> IDHKSKYLREAALEANLSHPETTPTMLTCPIDSGFLKDPVITPEGFVYNKSSILKWLETKKEDPQSRKPLTAKDLQPFPELLIIVNRFVETQTNYEKLKNRLVQNAR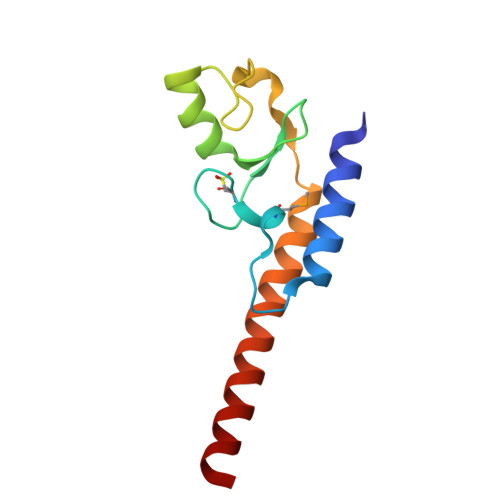VA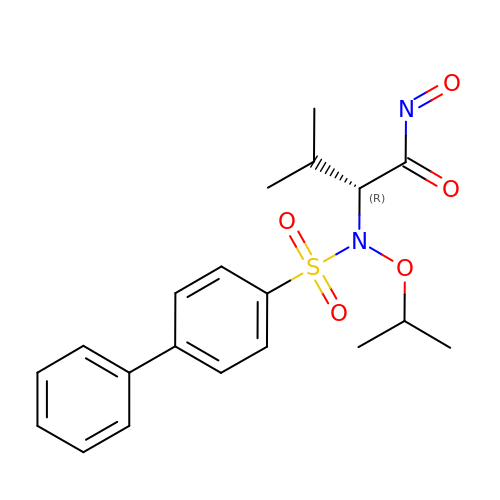(2~{R})-3-methyl-~{N}-oxidanylidene-2-[(4-phenylphenyl)sulfonyl-propan-2-yloxy-amino]butanamide | C20 H24 N2 O5 S | JYURKDGMICGTJM-LJQANCHMSA-N> HHHHHHASLRANDAPIVLLHGFTGWGREEMFGFKYWGGVRGDIEQWLNDNGYRTYTLAVGPLSSNW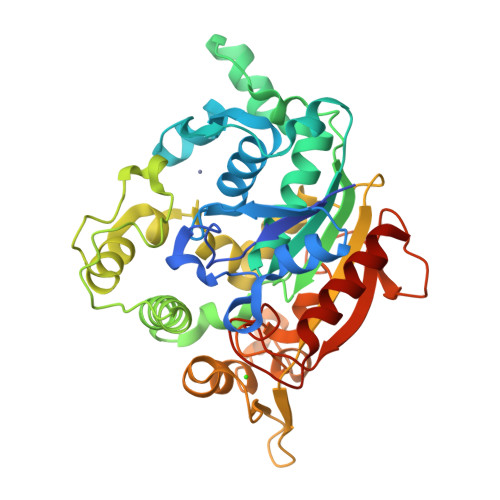DRACEAYAQLVGGTVDYGAAHAAKHGHARFGRTYPGLLPELKRGGRIHIIAHSQGGQTARMLVSLLENGSQEEREYAKAHNVSLSPLFEGGHHFVLSVTTIATPHDGTTLVNMVDFTDRFFDLQKAVLEAAAVASNVPYTSQVYDFKLDQWGLRRQPGESFDHYFERLKRSPVWTSTDTARYDLSVSGAEKLNQWVQASPNTYYLSFSTERTYRGALTGNHYPELGMNAFSAVVCAPFLGSYRNPTLGIDDRWLENDGIVNTVSMNGPKRGSSDRIVPYDGTLKKGVWNDMGTYNVDHLEIIGVDPNPSFDIRAFYLRLAEQLASLLP> GPLGSEDDLYRQSLEIISRYLREQATGSKDSKPLGEAGAAGRRALETLRRVGDGVQRNHETAFQGMLRKLDIKNEDDVKSLSRVMIHVFSDGVTNWGRIVTLISFGAFVAKHLKTINQESCIEPLAESITDVLVRTKRDWLVKQRGWDGFVEFFHVEDLEGG;>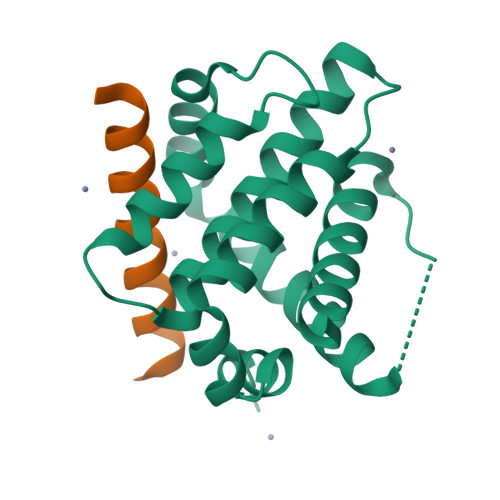 DMRPEIWIAQEARRIGDEANAYYARR> MELKHSISDYTEAEFLQLVATICDADATSEEELDKLITHFGEMTEHPSGSD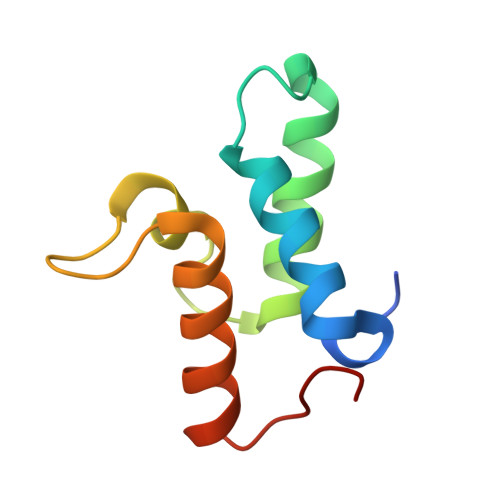LIYYPEEGDDDSPSGIVNTVKQWRAANGKSGFKQG> GPHMATGQDRVVALVDMDCFFVQVEQRQNPHLRNKPCAVVQYKSWKGGGIIAVSYEARAFGVTASMWADDAKKLCPDLLLAQVRESRGKANLTKYREASVEVMEIMSRFAVIERASIDEAYVDLTSAVQERLQKLQGQPISADLLPSTYIEGLPQGPTTAEETVQKEGMRKQGLFQWLDSLQIDNLTSPDLQLTVGAVIVEEMRAAIERETGFQCSAGISHNKVLAKLACGLNKPNRQTLVSHGSVPQLFSQMPIRKIRSLGGKLGASVIEILGIEYMGELTQFTESQLQSHFGEKNGSWLYAMCRGIEHDPVKPRQLPKTIGCSKNFPGKTALATREQVQWWLLQLAQE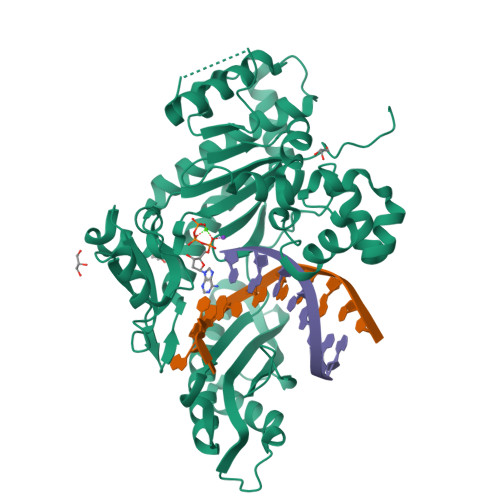LEERLTKDRNDNDRVATQLVVSIRVQGDKRLSSLRRCCALTRYDAHKMSHDAFTVIKNCNTSGIQTEWSPPLTMLFLCATKFSAS> VLGLAKLVG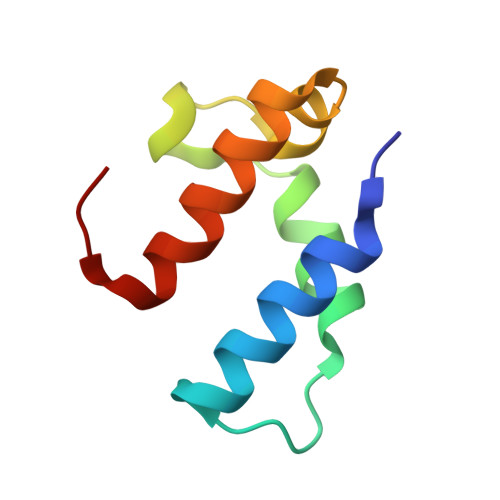QLEDMVEESGETDGFDAPEWLSSWLRQPLPALGGVNPIDLLDTMEGQAVVSRALAQIQSGAFA Peptidyl-tRNA hydrolase (Pth) hydrolyzes the ester bond between the peptide and the tRNA of peptidyl-tRNA molecules, which are the products of aborted translation, to prevent cell death by recycling tRNA. Pth releases the tRNA from the peptidyl-tRNA, by cleaving the ester bond between the C-terminal end of the peptide and the 2′- or 3′-hydroxyl group of the adenosine at the 3′-end of the tRNA (A76), and makes the free tRNA available for further rounds of protein synthesis. Pth1 adopts an α/β globular structure and functions as a monomeric enzyme, while Pth2 has a structure similar to thioredoxin and acts as a homodimeric enzyme. Here, we present the crystal structure of Thermus thermophilus Pth (TtPth) in complex with adenosine 5′-monophosphate (AMP), a mimic of A76.

To elucidate the binding mode of the peptidyl-A76 moiety of the substrate, we first determined the structure of TtPth in a complex with AMP by X-ray crystallography. The asymmetric unit of the crystal contains two TtPth⋅AMP complexes (A and B chains) and one AMP-unbound TtPth (C chain). The structures of the two TtPth⋅AMP complexes are quite similar (root mean square deviation for equivalent Cα atoms is 0.38 Å). The structure of TtPth⋅AMP revealed that AMP is bound to an acidic pocket at the bottom of the active site cleft (A−C). In this pocket, TtPth interacts with AMP via 9 amino acid residues (His19, Asp82, Glu83, Met84, Ala100, Gly101, Asn102, Arg103, and Ala134). Furthermore, the N6 atom of adenine forms hydrogen bonds with the side chain carboxyl oxygen of Glu83 and the main chain carbonyl oxygen of Ala100, and the N1 atom of adenine forms a hydrogen bond with the main chain amide nitrogen of Met84. In addition, the hydroxyl O2′ atom of the ribose hydrogen bonds with the main chain amide nitrogen of Arg103. No interaction was observed with the phosphate moiety of AMP. These results indicate that TtPth interacts primarily with the adenine and ribose moieties of AMP, while the phosphate moiety is minimally engaged by TtPth. Likewise, the distances between the gate loop (Asn102) and the lid loop (Val137) in TtPth⋅AMP and apo TtPth are 10.39 Å and 11.03 Å, respectively. These results indicate that AMP binding does not change the structure appreciably. In this research, the structure of the TtPth⋅AMP complex revealed that the adenine ring of the A76-mimicking AMP binds to the acidic pocket in the active site cleft.

>[3x]GSHMMFLVVGQGNPGERYARTRHNLGFMVLDRLGLSFRPRGEALVAEAEGGLFLKPLTYYNLTGRAVAPLARFYKIPPERILVVHDEMDLPLGRIRFKAGGSAAGNRGVLSIEEALGTRAFHRLRLGIGKPPDPSRGAEYVLSPFREEELPVVERVLEAAKEAVWCWVREGLPPCAGRFNGLDLSLG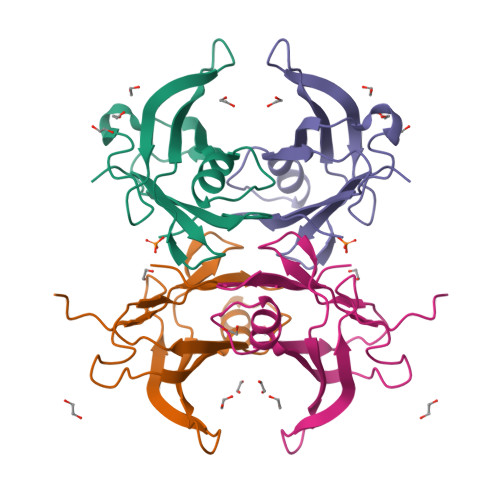>[2x]GHTAMASSESPLTTHVLNVAMGVPASNVTLRLYRQDPSSKTWQLLNTGITNEDGRYPGLITKELFTAGVYKLHFETAQYWASLGDTSFYPYVEIVFTINDPGQKYHVPLLLSRFSYSTYRGS>[2x]GMKLPRFGVEEWLNVHENSAIYDIAGVSISSLTLEELFALSGTNPEDFYKKLQGTKLNYGWIEGSPAFKKSVSQLYTGVKPEQILQTNGATGANLLVLYSLIEPGDHVISLYPTYQQLYDIPKSLGAEVDLWQIEEENGWLPDLEKLRQLIRPTTKMICINNANNPTGAVMDRTYLEELVEIASEVGAYILSDEVYRSFSELDVPSIIEVYDKGIAVNSLSKTYSLPGIRIGWVAANHQVTDILRDYRD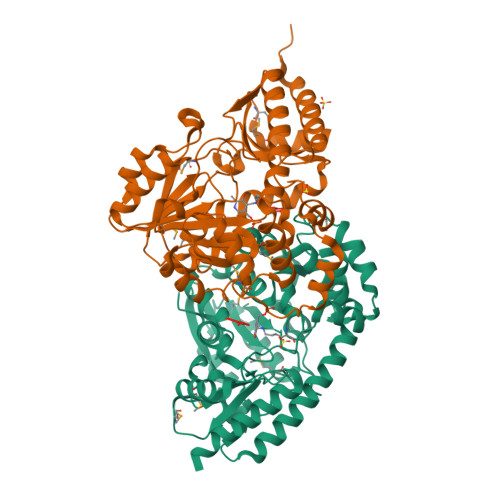YTMICAGVFDDLVAQLALAHYQEILERNRHILEENLAILDQWIEEEPLVSYIRPAVVSTSFVKIAVDMPMEDFCLQLLQEHGVLLVPGNRFERDGYVRLGFACEQETLIKGLEKLSQFLRRFDKEN> AKLRQFYVAAQSIRWNYRPESTHLSSKPFETSFKKIVYREYEAYFQKEKPQSRTSGLLGPTLYAEVGDIMKVHFKNKAHKPLSIHAQGIKYSKFSEGASYSDHTLPMEKMDDAVAPGQEYTYEWIISEHSGPTHDDPPCLTHIYYSYVNLVEDFNSGLIGPLLICKKGTLTEDGTQKMFEKQHVLMFAVFDESKSWNQTSSLMYTVNGYVNGTMPDITVCAHDHISWHLIGMSSGPELFSIHFNGQVLEQNHHKISAITLVSAT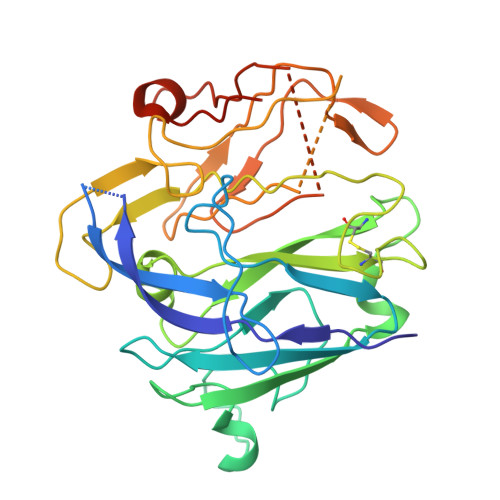STTANMTVSPEGRWTIASLIPRHFQAGMQAYIDIKNCAKKTR>[4x]DYLRELLKLELQAIKQYEKLRQTGDELVQAFQRLREIFDKGDDDSLEQVLEEIEELIQKHRQLASELPKLELQAIKQYREALE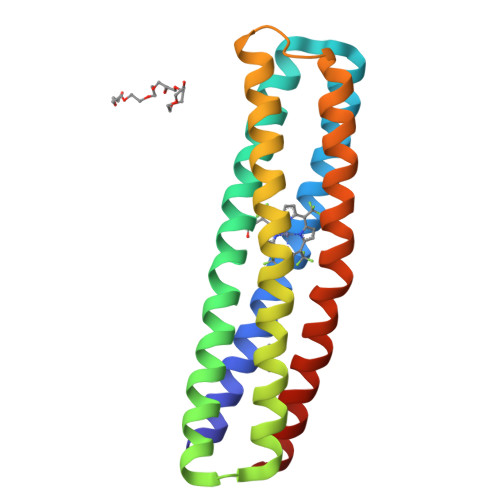YVKLPVLAKILEDEEKHIEWLKEAAKQGDQWVQLFQRFREAIDKGDKDSLEQLLEELEQALQKIRELTEKTGRKILEDEEKHIEWLETILG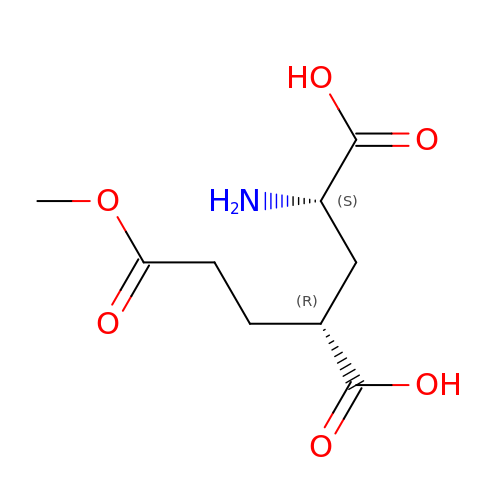(2S,4R)-4-(3-Methoxy-3-oxopropyl) glutamic acid | C9 H15 N O6 | IPTIKQIFOOZKAT-RITPCOANSA-N> MGHHHHHHSGQRKRGRQSKDEQLASDNELPVSAFQISEMSLSELQQVLKNESLSEYQRQLIRKIRRRGKNKVAARTCRQRR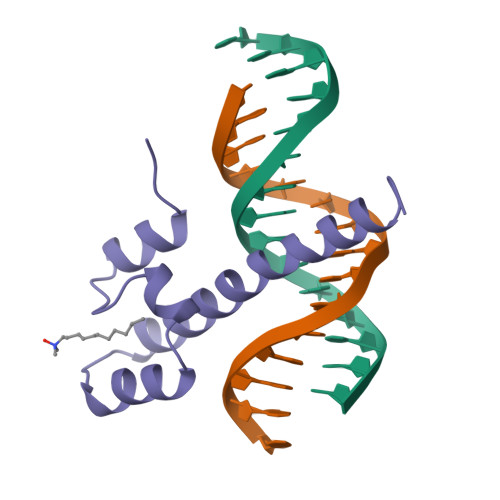TDRHDKMSHYI>MRVGLVGWRGMVGSVLMQRMVEERDFDLIEPVFFSTSQIGVPAPNFGKDAGMLHDAFDIESLKQLDAVITCQGGSYTEKVYPALRQ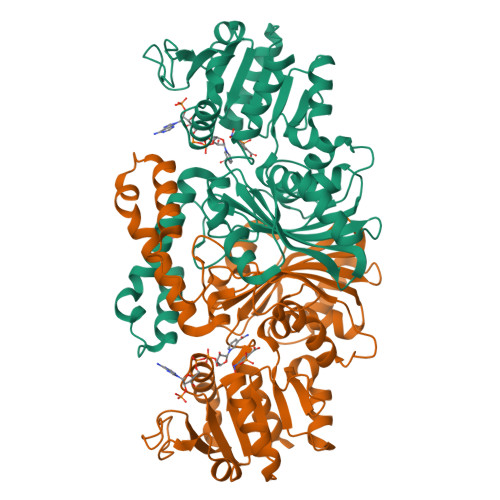AGWKGYWIDAASTLRMDKEAIITLDPVNLKQILHGIHHGTKTFVGGNCTVSLMLMALGGLYERGLVEWMSAMTYQAASGAGAQNMRELISQMGVINDAVSSELANPASSILDIDKKVAETMRSGSFPTDNFGVPLAGSLIPWIDVKRDNGQSKEEWKAGVEANKILGLQDSPVPIDGTCVRIGAMRCHSQALTIKLKQNIPLDEIEEMIATHNDWVKVIPNERDITARELTPAKVTGTLSVPVGRLRKMAMGDDFLNAFTVGDQLLWGAAEPLRRTLRIILAEKHHHHHH[2x]> SNAPYFGRPSLKTR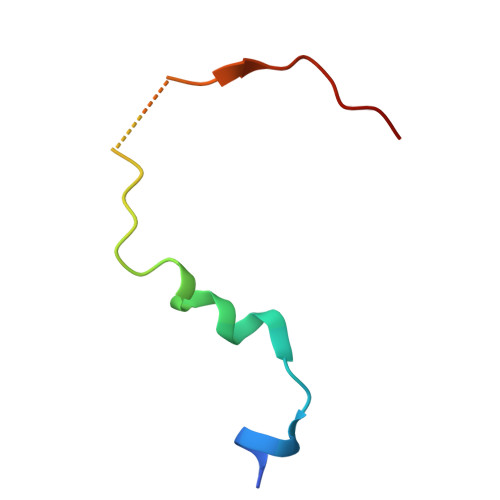AKQFEGVSSKDIGENCRRIEAFSD3-fluoro-4-nitrophenol | C6 H4 F N O3 | 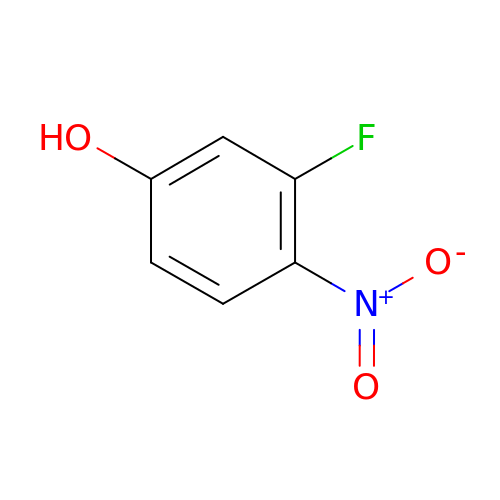CSSGKHVRDGATJL-UHFFFAOYSA-N> GSHMRKIQRYVRKDGKCNVHHGNVREKRAETLVFSTHAVISMRDGKLCLMFRVGDLRNSHIVRASIRAKLIKSKQTSEGEFIPLNQTDINVGYYTGDDRLFLVSPLIISHEINQQSPFWEISKAQLPKEELEIVVILEGMVEATGMTCQARSSYITSEILWGYRFTPVLTLEDGFYEVDYNSFHETYETSTPS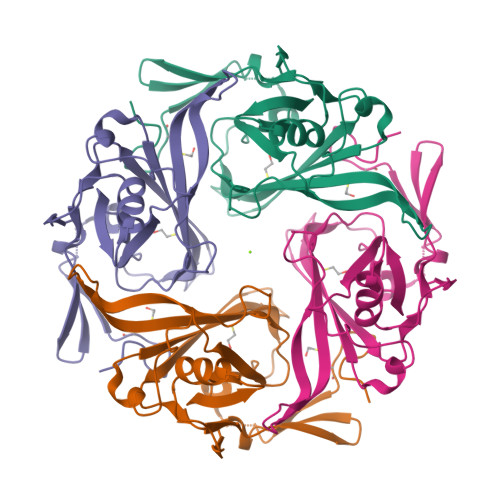LSAKELAELANRAEL>SNAMRDLKRHALFDPLTEALNRRGCEQAMRDSV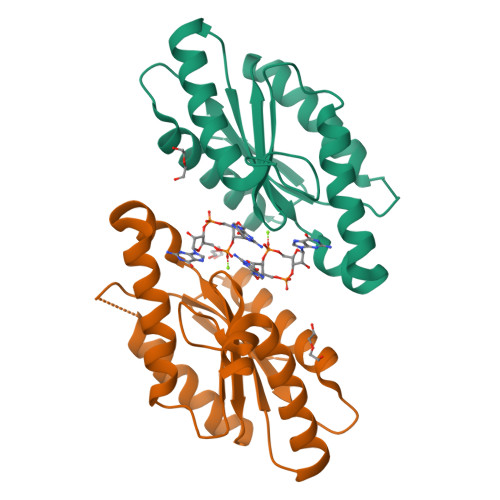TAAQREGWPFVLFVLDMDNLKPINDRFGHLAGDRVLVRLVESAYGWLGAQDWIGRWGGDEFLIGVHASEDEATLKLNQWLSMLEREDAEEAPLHVSAGSAVCEVGIDATELYRRADAAMYRAKFSGGRRLVRDG[2x]> VDCSEYPKPACTVEYRPLCG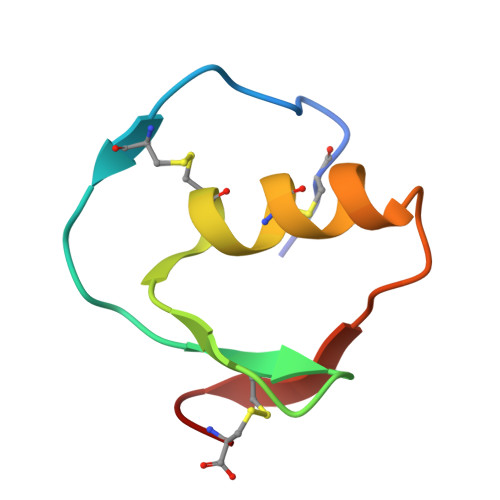SDNKTYGNKCNFCNAVVESNGTLTLSHFGKC Human DGCR8 is composed of an N-terminal region that is required for nuclear localization, a central heme-binding domain (HBD, residues 276–498), two double-stranded RNA-binding domains (dsRBDs, residues 500–700) and a C-terminal tail (CTT, residues 701–751). The HBD is a dimer and each HBD dimer binds one heme molecule. The HBD coordinates the heme Fe(III) using two thiol/thiolate groups from the highly-conserved Cys352 residues contributed by both subunits. The dimerization domain is an integral part of the heme-binding domain in human DGCR8; it aligns residues important for heme-binding in proper spatial positions.

We present the crystal structure of the frog (X. laevis) DGCR8 dimerization domain. Crystallographic refinement was performed using a model containing DGCR8 residues 300–355 and water molecules, and resulted in final R and Rfree factors of 0.2068 and 0.2280, respectively. Thus, our crystals contained the dimerization domain generated through degradation of the HBD. The frog dimerization domain crystal contains a single polypeptide chain in the asymmetric unit. The chain forms a dimer via a crystallographic twofold symmetry. After strand β3, the polypeptide chain extends through a hinge loop into a fourth β-strand (β4) that interacts with the WW motif of the partner subunit, forming a continuous β-sheet and resulting in an apparently domain-swapped dimer. All DGCR8 residues known to be important for heme binding, including Pro351, Cys352 and Trp329, cluster on a common surface. The dimerization domain structure of frog DGCR8 is very similar to that of human DGCR8 with some differences at the N- and C-termini. In the structural superimposition, the side chain of frog Cys354 points toward a direction distinct from that of human Cys352, as supported by a relatively weak but substantial electron density. Overall, the high degree of sequence and structural conservation suggests that frog DGCR8 uses the same mechanism of dimerization to aid heme binding as identified in human DGCR8.

> PPTEPLPDGWIMTFHNSGLPVYLHRETRVVTWSRPYFLGTGSIRKHDPPISSIPCL>[3x]GPLGSANPFSCKTNVCWAKALEPILATAGIVLTGCQWSELFPQFADDKPHSAIYALDVICIKFFGMDLTSGLFSKQSIPLTYHPADSARPVAHWDNSPGTRKYGYDHAIAAELSRRFPVFQLAGKGTQLDLQTGRTRVISAQHNLVPVNRNLPHALVPEYKEKQPGPVKKFLNQFKHHSVLVVSEEKIEAPRKRIEWIAPIGIAGADKNYNLAFGFPPQARYDLVFINIGTKYRNHHFQQCEDHAATLKTLSRSALNCLNPGGTLVVKSYGYADRNSEDVVTALARKFVRVSAARPDCVSSNTEMYLIFRQLDNSRTRQFTPHHLNCVISSVYEGTRDGVGAAPSYRTKRENIADCQEEAVVNAANPLGRPGEGVCRAIYKRWPTSFTDSATETGTARMTVCLGKKVIHAVG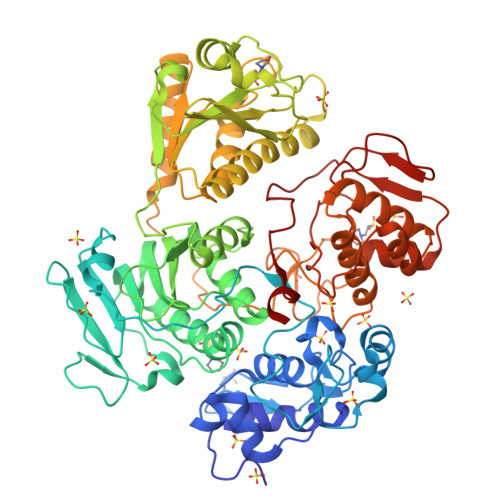PDFRKHPEAEALKLLQNAYHAVADLVNEHNIKSVAIPLLSTGIYAAGKDRLEVSLNCLTTALDRTDADVTIYCLDKKWKERIDAALQLKESVTELKDEDMEIDDELVWIHPDSCLKGRKGFSTTKGKLYSYFEGTKFHQAAKDMAEIKVLFPNDQESNEQLCAYILGETMEAIREKCPVDHNPSSSPPKTLPCLCMYAMTPERVHRLRSNNVKEVTVCSSTPLPKHKIKNVQKVQCTKVVLFNPHTPAFVPARKYIEV> MDHAEENEILAATQRYVVERPVYSQELLEEELEKKDRVPKTLGDKLKKSFRCSPKKAKNLLLSFFPILEWLPKYNLKEWLLGDLIAGLTVGSLQIPQGIAFALLAGLPPIYGLYSSFFPPLIYAFFGTSRHISVGPFAVVSLLVGSVVERLVPDDIVLPGGVNATNGTEARDALRVQVAFTLTFLAGIIQLALGLLRLGFLVDFLSEPLISGFTTGAAIHILLSQLKYLLGLKIPRHSGPFSVIYSVISVFHNIPNTNIATLGVSLLSFVLLLVVKELNKRFKKKLPVPIPAELIVVILATLISYYFNLAEKYGVSIVGHIPKGLPPPSVPDLSLFPLVIGDAIAIAIVGLAVSISVGKTFAKKHGYQIDGNQELIALGLMNIVGSFFSCYPATGSFSRSAVNESAGGKTQVAGIVAALVVLLVLLFLGPLFYYLPKAVLAAIIIVNLKGLLMQFKDAPKLWKVDKLDFLIWLVTFLGVVFLSVEIGLLVGVGFSLLTVLLRTQRPRTSVLGRIPGTDIYRDVKQYPEAEEVPGVKIFRIDSPIYFANSEYFKERLKRKTGVDPVKVLAARKKALKKIEKEIKKANLANKTVVKADAEVDGEDATKPEEEDGEVKYPPIVIQSDWPSELPRFVPPKVDFHTLILDFSAVSFVDTVGVKTLKEIVKEYREIGVQVYLAGCNASVVEKLERGGFFDDGITKEHLFLSVHDAVLFAQARKALAEQEASAPPSQEDLEPNATPATPEAGTENLYFQG

Prestin (SLC26A5) is abundantly expressed in the lateral membrane of OHCs, where it is responsible for electromotility. Prestin is unique in that it directly converts changes in the transmembrane electric potential into mechanical displacements. The structure of PresTS protein forms a domain-swapped homodimer, with each protomer consisting of 14 transmembrane (TM) α-helices and the C-terminal cytosolic Sulfate Transporter and Anti-Sigma factor antagonist (STAS) domain crossing each other. The TM domain is divided into two subdomains: the core (TM helices 1–4 and 8–11) and the gate (TM helices 5–7 and 12–14) domains.

The interdomain interface contains mostly hydrophobic residues. These structural observations indicate that the TM domain of the prestin protomer adopts the typical inverted repeat transporter fold, which presently adopts an inward-open conformation. The amino-terminal ends of the symmetrically arranged unwound helices (TM3 and TM10) are oriented toward this site, creating an electrically favorable environment for capturing negatively charged substrates between the dipoles. In fact, we observed a density at this site, probably corresponding to the Cl− ion stabilized in this position by R399 and S396. It is likely that F137 contributes to confining the Cl− ion at the site. Notably, the coordination distance between the Cl− ion, and R399 found in our cryo-EM PresTS structure is 4.49 Å, which is longer than the typical coordination distances of Cl− ions found in Cl−-bound protein structures deposited in the PDB server. The result revealed that the contribution from the helix dipole moments is larger than that by R399 (details in the legend), explaining the large coordination distance of the Cl− ion in the cryo-EM structure and in the simulations. The Q97, N447, and E293 residues participate in hydrogen-bonding interactions between the gate and core domains (Cl−-bound PresTS), while this interdomain interaction collapses upon the transition toward the Cl−-occluded state as captured in the recent prestin structures. A pivotal hydrophobic interface formed by V499 and I500 (mutated to leucine in PresTS) is located at the C-terminus of the long TM14 helix and involved in the domain-swapped dimerization interface of prestin. We also observed strong densities of lipid acyl chains and cholesterols on the gate domains, further suggesting the importance of their stabilization.FNR is a flavoenzyme that contains a noncovalently bound flavin adenine dinucleotide (FAD) as a prosthetic group. It catalyzes redox reactions between Fd and NAD(P)H. The redox-active component is the isoalloxazine ring of FAD, which undergoes transitions among three states: fully oxidized (FAD), semiquinone (; partially reduced) and hydroquinone (FADH2; fully reduced). In root plastids, which lack PS I, R-FNR reduces nonphotosynthetic Fd by oxidizing NADPH from the oxidative pentose phosphate pathway.

Previous X-ray structural studies of oxidized FNR have not accounted for the potential partial reduction caused by X-ray irradiation. To limit the reduction rate to less than 10%, it was necessary to keep the X-ray dose below 0.11 MGy. Consequently, X-ray diffraction data for wtFNRoxi crystals were collected using multiple irradiation points within a single crystal to minimize the dose. The absorbed dose during the diffraction experiment was calculated using RADDOSE-3D and estimated to be 0.097 MGy, meeting the required threshold. The X-ray structures of wild-type FNR in oxidized and reduced states were refined to 1.15 and 1.10 Å resolution, respectively, revealing no large structural changes in the main-chain backbones. The root-mean-square deviation (r.m.s.d.) of Cα atoms (residues 9–317) between wtFNRoxi and wtFNRred was 0.121 Å, indicating minimal structural differences at the backbone level. However, the Fo(wtFNRoxi) − Fo(wtFNRred) difference map revealed subtle but significant changes localized around the FAD/FADH2 moiety, highlighting the structural impact of FAD reduction.

> SRSKVSVAPLHLESAKEPPLNTYKPKEPFTATIVSVESLVGPKAPGETCHIVIDHGGNVPYWEGQSYGVIPPGENPKKPGAPQNVRLYSIASTRYGDNFDGRTGSLCVRRAVYYDPETGKEDPSKNGVCSNFLCNSKPGDKIQLTGPSGKIMLLPEEDPNATHIMIATGTGVAPFRGYLRRMFMEDVPNYRFGGLAWLFLGVANSDSLLYDEEFTSYLKQYPDNFRYDKALSREQKNRSGGKMYVQDKIEEYSDEIFKLLDGGAHIYFCGLKGMMPGIQDTLKKVAERRGESWDQKLAQLKKNKQWHVEVY> MGSIIFLEDRAFQGRIYGCTTDCPNLQPYFSRCNSIVVQSGCWMIYERPNYQGHQYFLRRGEYPDYQQWMGLSDSIRSCCLIPPHSGAYRMKIYDRDELRGQMSELTDDCLSVQ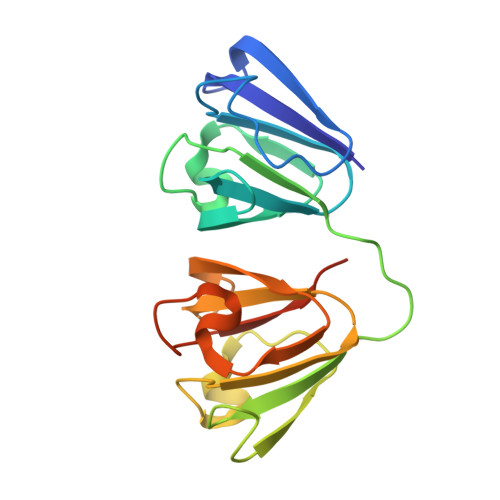DRFHLTEIHSLNVLEGSWILYEMPNYRGRQYLLRPGEYRRFLDWGAPNAKVGSLRRVMDLYLEHHHHHH> MASTSTGLPPNWTIRVSRSHNKEYFLNQSTNESSWDPPYGTDKEVLNAYIAKFKNNGYKPLVNEDGQVRVSH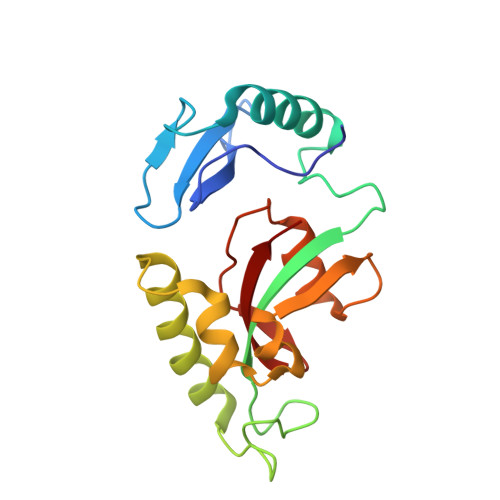LLIKNNQSRKPKSWKSPDGISRTRDESIQILKKHLERILSGEVKLSELANTESDCSSHDRGGDLGFFSKGQMQPPFEEAAFNLHVGEVSNIIETNSGVHILQRTG>MRGSHHHHHHGSLLIDKTVIVTGASRGIGRAAARECARQGARVVIGHSGSDEGRAGALSLAEEIAAF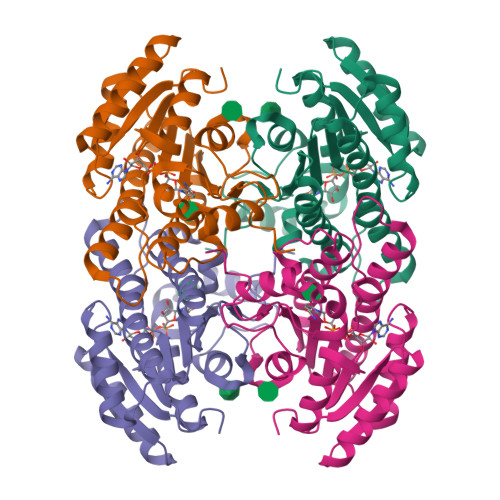GGTAIAVGADAADLDSGEKLVAAAVEAFGSVDVLVNNAGICPFHSFLDMPRELYLKTVGTNLNGAYFTVQAAARRMKEQGRGGAIIAVSSISALVGGAMQTHYTPTKAGLLSLMQSCAIALGPYGIRCNAVLPGTIATDINKEDLSDLEKRERMTSRVPLGRLGEPDDLAGPIVFLASDMARYVTGASLLVDGGLFVNLQ[2x]>LSPDAYRFLTEQDRQLRLEQAQIQRLLEAQSL[6x]

Here, we probe the mechanism of oligomerization of a peptide representing the CCD of the STIL protein, a tetrameric multi-domain protein that is over-expressed in several cancers and associated with metastatic spread. STIL tetramerization is mediated both by an intrinsically disordered domain (STIL400–700) and a structured CCD (STIL CCD718–749). The STIL protein plays a highly important role in mitosis by regulating centrosomal duplication. The CCD of STIL is necessary for its self-association.

Our previous studies of the isolated STIL CCD domain (STIL CCD peptide) have shown that a single Leu-to-Glu substitution at position 736, a d site of the predicted CC repeat in the STIL CCD peptide, leads to a decrease in its thermal stability. Presumably, this is due to the disruption of the hydrophobic CC interactions upon mutation from the hydrophobic Leu to the charged Glu. Indeed, expression of the full-length L736E mutant in Stil−/− mouse embryonic fibroblasts completely disrupts the formation of centrosomes and cilia compared to WT STIL, which rescues this phenotype. AUC-SV measurements at 10 µM and 500 µM of the CCD718–749-L736E peptide returned an oligomeric state of 1 × monomer mass. No detectable change in the Tm at different L736E concentrations was observed. These data are all consistent with the L736E mutation destabilizing the proposed oligomerization of the CCD peptide leading to a folded monomer in solution without the additional stability measured for the WT CCD. The L736E peptide formed an antiparallel dimer in the crystal state. The structure has hydrophobic side chains in the tight dimer interface, which the program SOCKET2 identifies as an antiparallel coiled coil with typical knobs-into-holes interactions. However, there are fewer exposed hydrophobic residues that might be expected for the peptide to form a tetramer interface previously predicted by us and presented by others. Helical-wheel projections for one heptad repeat of the L736E mutant indicate the potential disruption that would be caused by placing Glu-736 between the helices of the putative tetramer. This may explain the monomeric state measured by the AUC-SV in solution.OGA is the unique enzyme responsible for O-GlcNAc hydrolysis from a large number of cytoplasmic and nuclear proteins. Recently, our group and others have independently identified crystallizable constructs of OGA that comprise the catalytic domain and stalk domain, and published the apo form structures and enzyme complexes with active site inhibitors. These reports consistently showed that OGA formed an unusual arm-in-arm homodimer, where the catalytic domain of one monomer covered by the stalk domain of the sister monomer to create a potential substrate-binding cleft. Exploiting our previously reported construct of OGAcryst (residues 60–704 with the unstructured insert residues 401–552 replaced by a glycine–serine (GS) linker), we solved the structures of a mutant OGAcryst-D175N (catalytically impaired but retaining the ability to bind substrate) in apo form and in complex with each of four synthetic glycopeptides.

In the substrate complexes, all the glycopeptides were bound in the OGA substrate-binding cleft. Particularly, the GlcNAc moieties were anchored by the same set of OGA residues in the catalytic pocket, displaying nearly identical binding conformations regardless of the glycosylated residues or the flanking peptide sequences. Consistent with the O-GlcNAc hydrolysis mechanism, the catalytic residue D174 was optimally positioned to make a hydrogen bond with the N-acetyl group of GlcNAc in all the complexed structures. The N175 mutant side chain played an important role in anchoring the glycosylated hydroxyl of serine or threonine and stabilizing the OGA substrate complexes. Compared to the glycosylated serine, the extra methyl group of the glycosylated threonine (as found in ELK1 and Lamin B1 peptides in Fig. 2c, d) was well accommodated in the hydrophobic pocket harboring F223 and V254 residues from the top surface of the catalytic domain and W679 from the stalk domain of the sister monomer. In the structure of OGA-ELK1 complex, residues Y69 and N175 anchored the peptide backbone. Furthermore, side chain specific interactions with cleft surface residues reinforced the binding. We find that OGA is able to bind peptide substrates in different directions, but in a conserved conformation regardless of the glycosylation site or flanking sequences.

>[2x]HFLCGVVEGFYGRPWVMEQRKELFRRLQKWELNTYLYAPKDDYKHRMFWREMYSVEEAEQLMTLISAAREYEIEFIYAISPGLDITFSNPKEVSTLKRKLDQVSQFGCRSFALLFDNIDHNMCAADKEVFSSFAHAQVSITNEIYQYLGEPETFLFCPTEYCGTFCYPNVSQSPYLRTVGEKLLPGIEVLWTGPKVVSKEIPVESIEEVSKIIKRAPVIWDNIHANDYDQKRLFLGPYKGRSTELIPRLKGVLTNPNCEFEANYVAIHTLATWYKSNMNGVRKDVVMTDSEDSTVSIQIKLENEGSDEDIETDVLYSPQMALKLALTEWLQEFGVPHQYSSRGGGGSGGGGSVTLEDLQLLADLFYLPYEHGPKGAQMLREFQWLRANSSVVSVNCKGKDSEKIEEWRSRAAKFEEMCGLVMGMFTRLSNCANRTILYDMYSYVWDIKSIMSMVKSFVQWLGCRSHSSAQFLIGDQEPWAFRGGLAGEFQRLLPIDGANDLFFQ;>[2x]FWSTLSPI>[2x]EPGENLKPVDAMQCFDCHTQIEDMHTVGKHATVNCVHCHDATEHVETASSRRMGERPVTRMDLEACATCHTAQFNSFVEVRHESHPRLEKATPTSRSPMFDKLIAGHGFAFEHAEPRSHAFMLVDHFVVDRAYGGRFQFKNWQKVTDGMGAVRGAWTVLTDADPESSD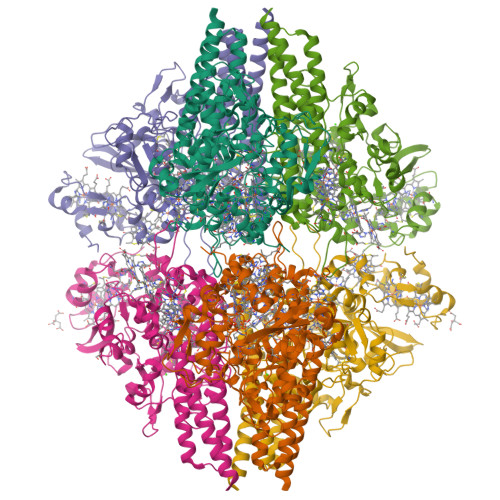QRRFLSQTATAANPVCLNCKTQDHILDWAYMGDEHEAAKWSRTSEVVEFARDLNHPLNCFMCHDPHSAGPRVVRDGLINAVVDRGLGTYPHDPVKSEQQGMTKVTFQRGREDFRAIGLLDTADSNVMCAQCHVEYNCNPGYQLSDGSRVGMDDRRANHFFWANVFDYKEAAQEIDFFDFRHATTGAALPKLQHPEAETFWGSVHERNGVACADCHMPKVQLENGKVYTSHSQRTPRDMMGQACLNCHAEWTEDQALYAIDYIKNYTHGKIVKSEYWLAKMIDLFPVAKRAGVSEDVLNQARELHYDAHLYWEWWTAENSVGFHNPDQARESLMTSISKSKEAVSLLNDAIDAQVASR> MSEHQSLPAPEASTEVRVAIVGVGNCASSLVQGVEYYYNADDTSTVPGLMHVRFGPYHVRDVKFVAAFDVDAKKVGFDLSDAIFASENNTIKIADVAPTNVIVQRGPTLDGIGKYYADTIELSDAEPVDVVQALKEAKVDVLVSYLPVGSEEADKFYAQCAIDAGVAFVNALPVFIASDPVWAKKFTDARVPIVGDDIKSQVGATITHRVLAKLFEDRGVQLDRTMQLNVGGNMDFLNMLERERLESKKISKTQAVTSNLKREFKTKDVHIGPSDHVGWLDDRKWAYVRLEGRAFGDVPLNLEYKLEVWDSPNSAGVIIDAVRAAKIAKDRGIGGPVIPASAYLMKSPPEQLP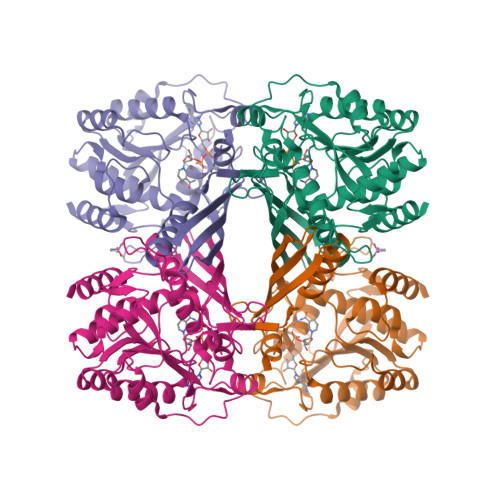DDIARAQLEEFIIG>[2x]VSVITSEMKMELRMEGAVNGHKFVITGK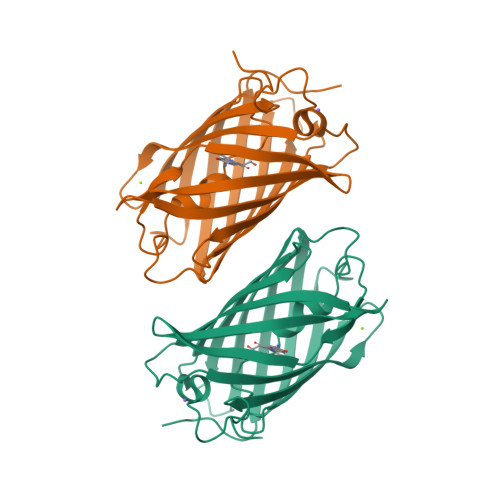GSGQPFEGIQNMDLTVIEGGPLPFAFDILTTVFDYGNRVFVKYPEEIVDYFKQSFPEGYSWERSMSYEDGGICLATNNITMKKDGSNCFVYEIRFDGVNFPANGPVMQRKTVKWEPSTEKMYVRDGVLKGDVNMALLLQGGGHYRCDFRTTYKAKKVVQLPDYHFVDHRIEITSHDKDYNKVKLYEHAKAHSGLPRLAK>GSSHHHHHHSSGLVPRGSHMKSTSVSPFHLPLNHPTYLIWSANTSLGKTLVSTGIAASFLLQQPSSSATKLLYLKPIQTGFPSDSDSRFVFSKLDSLSLRRQIPISISNSVLHSSLPAAKSLGLNVEVSESGMCSLNFRDEKTVTGAPELLCKTLYAWEAAISPHLAAERENATVEDSVVLQMIEKCLKEEMECGVKSEKSDLLCLVETAGGVASPGPSGTLQCDLYRPFRLPGILVGDGRLGGISGTIAAYESLKLRGYDIAAVVFEDHGLVNEVPLTSYLRNKVPVLVLPPVPKDPSDDLIEWFVESDGVFKALKETMVLANLERLERLNGMAKLAGEVFWWPYTQHKLVHQETVTVIDSRCGENFSIYKASDNSSLSQQFDACASWWTQGPDPTFQAELAREMGYTAARFGHVMFPENVYEPALKCAELLLDGVGKGWASRVYFSDNGSTAIEIALKMAFRKFCVDHNFCEATEEEKHIVVKVIALRGSYHGDTLGAMEAQAPSPYTGFLQQPWYTGRGLFLDPPTVFLSNGSWNISLPESFSEIAPEYGTFTSRDEIFDKSRDASTLARIYSAYLSKHLQEHSGVRQSAHVGALIIEPVIHGAGGMHMVDPLFQRVLVNECRNRKIPVIFDEVFTGFWRLGVETTTELLGCKPD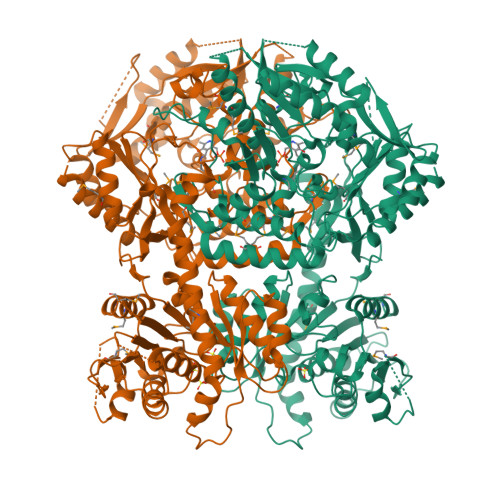IACFAKLLTGGMVPLAVTLATDAVFDSFSGDSKLKALLHGHSYSAHAMGCATAAKAIQWFKDPETNHNITSQGKTLRELWDEELVQQISSHSAVQRVVVIGTLFALELKADASNSGYASLYAKSLLIMLREDGIFTRPLGNVIYLMCGPCTSPEICRRLLTKLYKRLGEFNRT[2x]> GAMGEQIFYWSPAKHWRMSDEGVVIGESTYTGMILEWFPEFYFFAQTGVTINRLLERFSSGSEKEANEILELLIQDRVLVEGILPPREVFSPQEGLFVNPYSEQIRYSKEALDYYVSEQLNRTHAACRSTKIQLETSGALPDIIQKRRSCRRFDMKTPVSFATFSNLLSSLKQRKEDKILYNYASAGGLYPIDVFVYVKPRRVEGVKAGFYYFNPADHSLVLVNNIDQVIKDDHELINQDIFAQSAFSVYLVYNARASMPKYGAAGYFYACIEAGIITATLNMVAEDLNVGLCSIGHMNFEEIQTFLKLEDHQVILHAIEGGLKID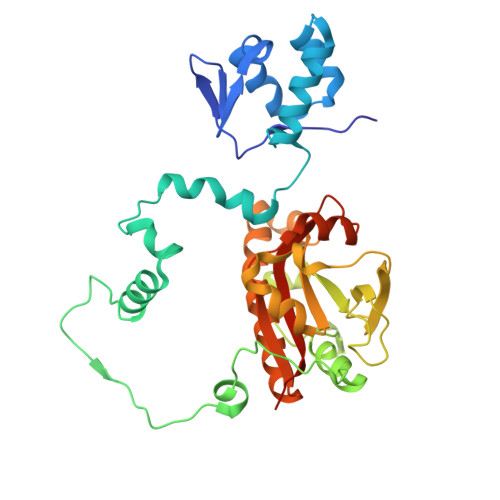GAAAENLYFQ>MFTTKLAEKVVSAWKAKISQPALKAAQDGVIDTVAAALGGVTEHSVQVALKYVAATGGSGDSKLWGVNQRSNMFDAAFVNGMAAHAIDFDDSFPVMRGHPSSSLVPAIFAVGEHVGANGHNCLKSYVLGIEVVATLGRAVGKGHYLAGWHPTSTLGVFGATTAAALLLGADEEQLRNAWGIAASNSCGIIKNFGTMTKPMHTGSAARNGVLSAWLSMQSFTGCQTVFDDAEGILAMYGAQPGPELFNAMQKFGTPWAI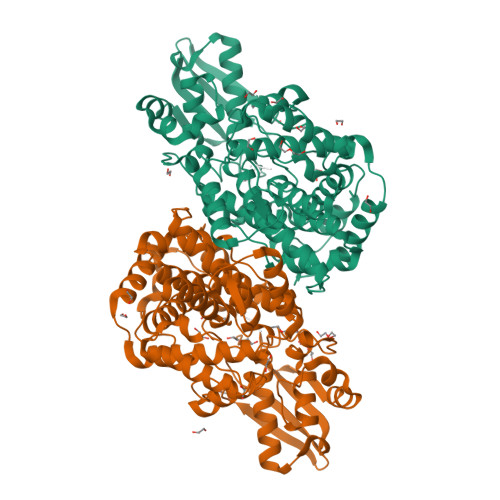IAPGLYKKSWPSCYANHKPLAGLFAIMKEHGLTGQDISHVDVGFLPGVEKPLLYMDPRTTEEAKFSIEANIGAALLDGEVSLASFEIEHLDRPAMRAAMKKVTRFDMPSETTFSGTTGYTDIVVHTADGKIERRIEATPGSLEDPMDDAHLERKFKDCTAWMPFGESGLLFDRLRSLTADQGIKTVQP[2x]TERT-BUTYL 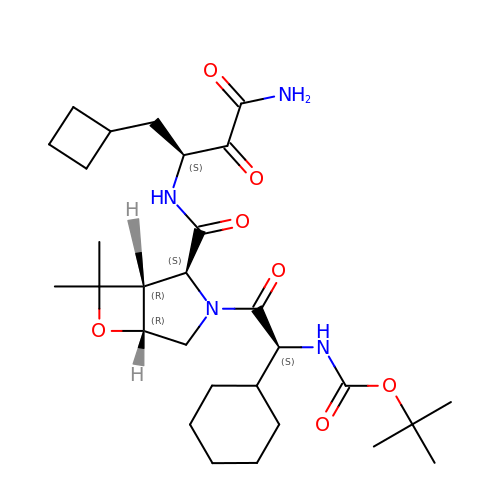{(1S)-2-[(1R,2S,5R)-2-({[(1S)-3-AMINO-1-(CYCLOBUTYLMETHYL)-2,3-DIOXOPROPYL]AMINO}CARBONYL)-7,7-DIMETHYL-6-OXA-3-AZABICYCLO[3.2.0]HEPT-3-YL]-1-CYCLOHEXYL-2-OXOETHYL}CARBAMATE | C29 H46 N4 O7 | WRVVRHORVNXEJF-YFNVTMOMSA-N> SPNSQYLKTRILDIYTPEQRAGIEKSEDWRQFSRRMDTHFPKLMNELDSVYGNNEALLPMLEMLLAQAWQSYSQRNSSLKDIDIARENNPDWILSNKQVGGVCYVDLFAGDLKGLKDKIPYFQELGLTYLHLMPLFKCPEGKSDGGYAVSSYRDVNPALGTIGDLREVIAALHEAGISAVVDFIFNHTSNEHEWAQRCAAGDPLFDNFYYIFPDRRMPDQYDRTLREIFPDQHPGGFSQLEDGRWVWTTFNSFQWDLNYSNPWVFRAMAGEMLFLANLGVDILRMDAVAFIWKQMGTSCENLPQAHALIRAFNAVMRIAAPAVFFKSEAIVHPDQVVQYIGQDECQIGYNPLQMALLWN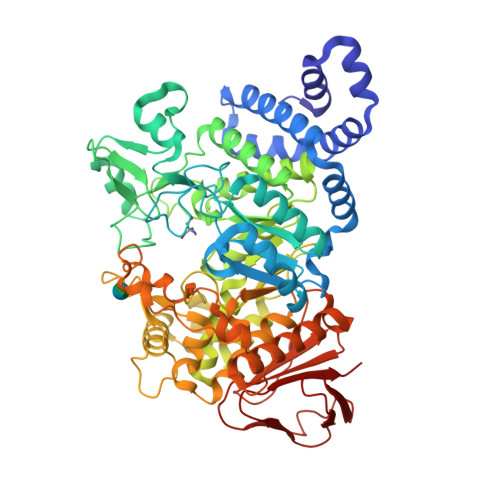TLATREVNLLHQALTYRHNLPEHTAWVNYVRSHDDIGWTFADEDAAYLGISGYDHRQFLNRFFVNRFDGSFARGVPFQYNPSTGDCRVSGTAAALVGLAQDDPHAVDRIKLLYSIALSTGGLPLIYLGDEVGTLNDDDWSQDSNKSDDSRWAHRPRYNEALYAQRNDPSTAAGQIYQDLRHMIAVRQSNPRFDGGRLVTFNTNNKHIIGYIRNNALLAFGNFSEYPQTVTAHTLQAMPFKAHDLIGGKTVSLNQDLTLQPYQVMWLEIA>MKRIGVLTSGGDSPGMNAAVRAVVRKAIYHDVEVYGIYNGYAGLISGKIEKLELGSVGDIIHRGGTKLYTARCPEFKTVEGREKGIANLKKLGIEGLVVIGGDGSYMGAKKLTEHGFPCVGVPGTIDNDIPGTDFTIGFDTALNTVIDAIDKIRDTATSHERTYVIEVMGRHAGDIALWAGLAGGAESILIPEADYDMHEIIARLKRGHERGKKHSIIIVAEGVGSGVEFGKRIEEETNLETRVSVLGHIQRGGSPSAADRVLASRLGAYAVELLLEGKGGRCVGIQNNKLVDHDIIEILETKHT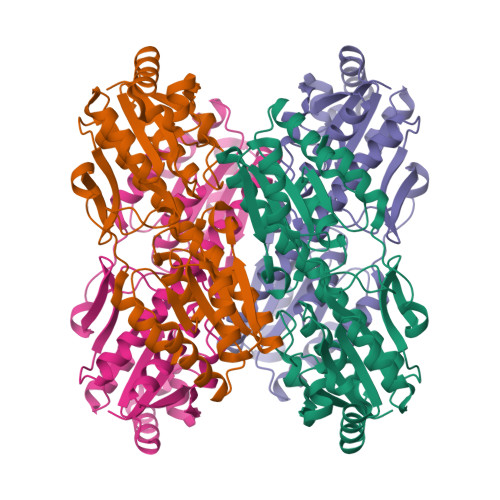VEQNMYQLSKELSI[2x]> MESKRLDNAALAAGISPNYINAHGKPQSISAETKRRLLDAMHQRTATKVAVTPVPNVMVYTSGKKMPMVVEGSGEYSWLLTTEEGTQYKGHVTGGKAFNLPTKLPEGYHTLTLTQDDQRAHCRVIVAPKRCYEPQALLNKQKLWGACVQLYTLRSEKNWGIGDFGDLKAMLVDVAKRGGSFIGLNPIHALYPANPESASPYSPSSRRWLNVIYIDVNAVEDFHLSEEAQAWWQLPTTQQTLQQARDADWVDYSTVTALKMTALRMAWKGFAQRDDEQMAAFRQ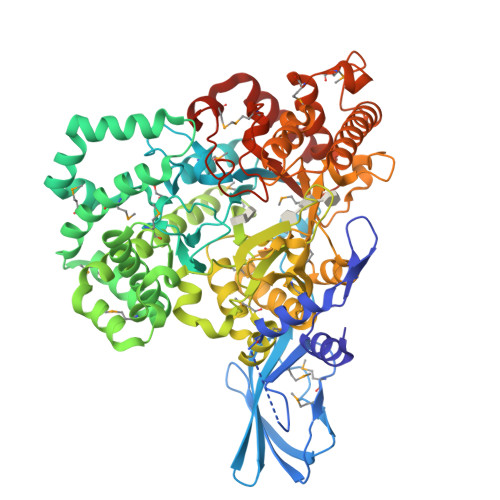FVAEQGDSLFWQAAFDALHAQQVKEDEMRWGWPAWPEMYQNVDSPEVRQFCEEHRDDVDFYLWLQWLAYSQFAACWEISQGYEMPIGLYRDLAVGVAEGGAETWCDRELYCLKASVGAPPDILGPLGQNWGLPPMDPHIITARAYEPFIELLRANMQNCGALRIDHVMSMLRLWWIPYGETADQGAYVHYPVDDLLSILALESKRHRCMVIGEDLGTVPVEIVGKLRSSGVYSYKVLYFENDHEKTFRAPKAYPEQSMAVAATHDLPTLRGYWECGDLTLGKTLGLYPDEVVLRGLYQDRELAKQGLLDALHKYGCLPKRAGHKASLMSMTPTLNRGLQRYIADSNSALLGLQPEDWLDMAEPVNIPGTSYQYKNWRRKLSATLESMFADDGVNKLLKDLDRRRRSAHHHHHH>[2x]GASLEHHHHHHENLYFQSGTRWAVLVAGSSGYWNYRHQADICHAYQLLRKGGLKEENIVVFMYDDIANNYENPRPGTIINSPHGKDVYQGVPKDYTGDDVNVDNLFAVILGDKTAVKGGSGKVVDSGPNDHIFIFYSNHGGPGVLGMPTSPYLYANDLNDVLKKKHALGTYKSLVFYLEACESGSIFEGLLPEGLNIYATTASNAEESSWGTYCPGEEPSPPPEYETCLGDLYSVAWMEDSGMHN;>[2x]LQTETLHQQYELVKRRTAPVGYSYGSHVMQYGDVGISKDNLDLYMGTNPAN

Arabidopsis thaliana encodes four legumain forms, two vegetative-type (AtLEGα and γ), one seed-type (AtLEGβ), and a separate grouped (AtLEGδ). The vegetative-type legumains, like AtLEGγ, are involved in plant-programmed cell death. Legumains are synthesized as inactive precursors, or zymogens, with a tripartite domain organization. It comprises an N-terminal asparaginyl endopeptidase domain (AEP),2 an intermediate activation peptide that blocks access to the active site and thus confers enzymatic latency to the zymogen, and a C-terminal legumain stabilization and activity modulation (LSAM) domain, which renders legumain stable at neutral pH and restricts substrate access to the active site.

For a detailed understanding of how fully activated A. thaliana legumain γ (AtLEGγ) recognizes a substrate, we solved the crystal structure of the AtLEGγ peptidase (AEP) in complex with the covalent peptidic CMK-based inhibitor Ac-YVAD-CMK to 1.5-Å resolution. The peptidase (AEP) exhibited the characteristic six-stranded central β-sheet (β1–β6), which was surrounded by five major and five minor α-helices. When we analyzed the AtLEGγ structure in complex with the Ac-YVAD-CMK ligand we found the specificity loops (c341 and c381) and the edge strand (βIV) highly ordered, contrasting the zymogenic structure, displayed in relative B-factors, which indicate the local flexibility. In the Ac-YVAD-CMK substrate analogue, there were two major hydrogen bonds between the carbonyl oxygen of Ser247 and amide nitrogen of Gly249 to P1 amide nitrogen and P2 carbonyl oxygen, respectively. The P2 carbonyl oxygen was further anchored by the side chain of Arg74. By contrast, the activation peptide in the two-chain structure was out of register and shifted for 2.5 Å to the N-terminal direction. The oxyanion hole was formed by the amide nitrogens of Cys219 and Gly178 as well as of imidazole ring of His177 (Nδ1). The protonated AspP1 carboxylate group was coordinated by Asp269 and Glu217 at the bottom, Ser247 on the upper side (“north”) and Arg74 and His75 on the lower side (“south”) of the S1 pocket. The P2 Ala interacted hydrophobically with Trp248. The P3 Val was constrained by the Cys252–Cys266 disulfide bridge and the guanidium group of Arg74.The second pathway involves the sterol-regulated inducible degrader of the LDLR (IDOL, also known as MYLIP), which is an E3 ubiquitin ligase that promotes the ubiquitylation and subsequent lysosomal degradation of the LDLR. Two distinct protein domains are present in IDOL: an N-terminal FERM (band 4.1/ezrin/radixin/moesin) and a C-terminal RING domain. In contrast to secreted PCSK9, which interacts with the LDLR extracellularly, IDOL is a 45-kDa cytoplasmic protein that interacts with the intracellular tail of the LDLR via its FERM domain. Here we present two crystal structures of the FERM domain of human IDOL.

The FERM344 protein crystallized in space group I4122, with unit-cell parameters a = b = 159.49 Å, c = 76.72 Å, α = β = γ = 90°, with one molecule in the asymmetric unit and a solvent content of 60%. The F1, F2, and F3 regions of FERM344 adopt the archetypical cloverleaf structure of the FERM domains. However, our structure shows that F3ab runs from 186 to 278 and that the region spanning residues 279–332 is clearly outside the cloverleaf region. Based on the obtained structure, we propose to redefine IDOL FERM boundaries as shown in Fig. 1A, with the extra region in FERM (which spans residues 279–344) divided into three subdomains to accentuate the extension away from the F3ab lobe: F3c′ (residues 279–300), F3c″ (residues 301–332), and F3c‴ (residues 333–344), with the latter not traceable in the electron density map. After the α7 helix, the FERM344 structure has a partially unstructured region from residue 301 until residue 317, followed by helix α8 (residues 318–332) (F3c″), which is the last residue traceable in the electron density map. Moreover, there are clear differences in the F3c′ region, where the FERM344 crystal structure has an α helix (α7), following the F3ab, which spans residues 279–300 and folds back onto the F3ab. The FERM344 domain packs as a tetramer in the crystal created by crystallographic symmetry operations. Its extended F3c′-F3c″ region (residues 279–332) interacts extensively with F1 and F3 of a symmetry-related molecule, burying a substantial surface area of 2537 Å2. In the FERM344 structure, the F3c′ is helical and positioned over the F3ab domain, obscuring the access to the peptide binding site. If this particular position is retained in full-length IDOL, it could prevent the interaction with the LDLR intracellular tail, suggesting a possible form of autoinhibition.

> GGMLCYVTRPDAVLMEVEVEAKANGEDCLNQVCRRLGIIEVDYFGLQFTGSKGESLWLNLRNRISQQMDGLAPYRLKLRVKFFVEPHLILQEQTRHIFFLHIKEALLAGHLLCSPEQAVELSALLAQTKFGDYNQNTAKYNYEELCAKELSSATLNSIVAKHKELEGTSQASAEYQVLQIVSAMENYGIEWHSVRDSEGQKLLIGVGPEGISICKDDFSPINRIAYPVVQMATQSGKNVYLTVTKESGNSIVLLFKMISTRAASGLYRAITETHAFYRCDTVTSAVMMQYSRDLKGHLASLFLNENINLGKKYVFDIKRTSKEVYDHARRALYNAGVVDLVSRNNQ>[2x]MINAIRTPDQRFSNLDQYPFSPNYLDDLPGYPGLRAHYLDEGNSDAEDVFLCLHGEPTWSYLYRKMIPVFAESGARVIAPDFFGFGKSDKPVDEEDYTFEFHRNFLLALIERLDLRNITLVVQDWGGFLGLTLPMADPSRFKRLIIMNACLMTDPVTQPAFSAFVTQPADGWTAWKYDLVTPSDLRLDQFMKRWAPTLT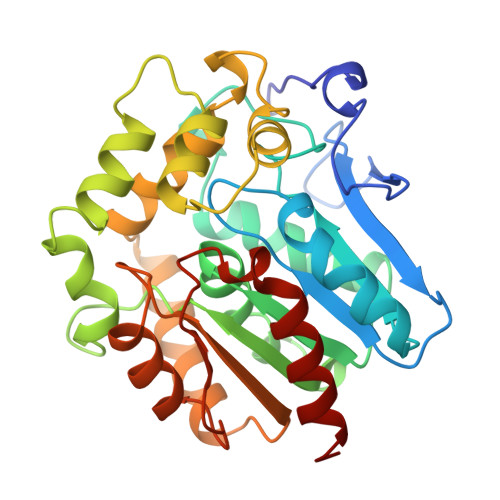EAEASAYAAPFPDTSYQAGVRKFPKMVAQRDQACIDISTEAISFWQNDWNGQTFMAIGMKDKLLGPDVMYPMKALINGCPEPLEIADAGHFVQEFGEQVAREALKHFAETE>MGFNVKTPLLATDVIIR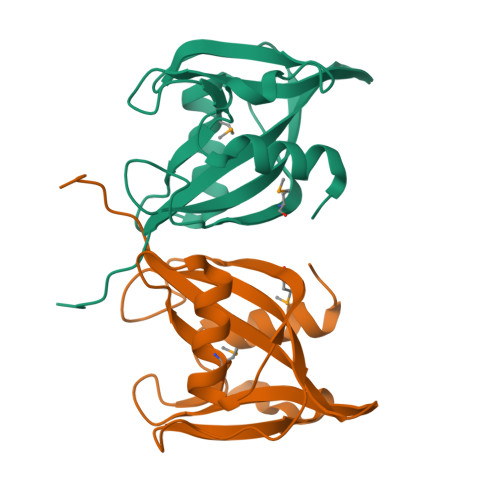LWDGENFKGIVLIERKYPPVGLALPGGFVEVGERVEEAAAREMREETGLEVRLHKLMGVYSDPERDPRAHVVSVVWIGDAQGEPKAGSDAKKVKVYRLEEIPLDKLVFDHKKIILDFLKGNY[4x]>SRVLLALHDRAPQLKISDDRLTVVGEKGYSMVRASHGVRKGAWYFEITVDEMPPDTAARLGWSQPLGNLQAPLGYDKFSYSWRSKKGTKFHQSIGKHYSSGYGQGDVLGFYINLPEDT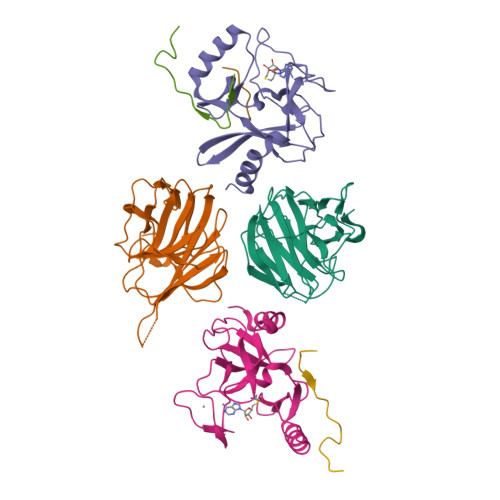ISGRGSSEIIFYKNGVNQGVAYKDIFEGVYFPAISLYKSCTVSINFGPCFKYPPKDLTYRPMSDMG[2x];>[2x]GPLGSKSSQYRKMKTEWKSNVYLARSRIQGLGLYAARDIEKHTMVIEYIGTIIRNEVANRKEKLYESQNRGVYMFRMDNDHVIDATLTGGPARYINHSCAPNCVAEVVTFERGHKIIISSSRRIQKGEELCYDYKFDFEDDQHKIPCHCGAVNCRKWMN;>[2x]SAFAPDFKELDENVEYEERESEFDIED;> ARTKQTARK>[2x]AAECSVDIQGNDQMQFNTNAITVDKSCKQFTVNLSHPGNLPKNVMGHNWVLSTAADMQGVVTDGMASGLDKDYLKPDDSRVIAHTKLIGSGEKDSVTFDVSKLKEGEQYMF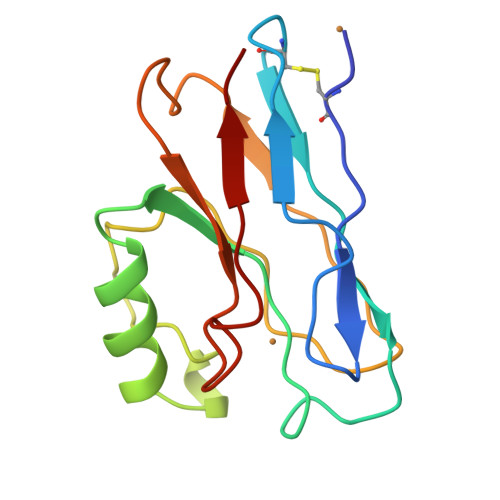FDTFPGHSALMKGTLTLK>MAGDTTITVVG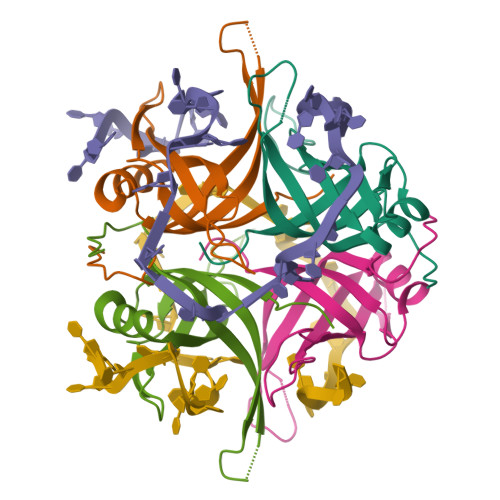NLTADPELRFTPSGAAVANFTVASTPRMFDRQSGEWKDGEALFLRCNIWREAAENVAESLTRGSRVIVTGRLKQRSFETREGEKRTVVEVEVDEIGPSLRYATAKVNKASRSGGGGGGF[2x]>[2x]MRVLGIETSCDETGIAIYDDEKGLLANQLYSQVKLHADYGGVVPELASRDHVRKTVPLIQAALKESGLTAKDIDAVAYTAGPGLEGALLVGATVGRSLAFAWDVPAIPVHHMEGHLLAPMLEDNPPEFPFVALLVSGGHTQLISVTGIGQYELLGESIDDAAGEAFDKTAKLLGLDYPGGPLLSKMAAQGTAGRFVFPRPMTDRPGLDFSFSGLKTFAANTIRDNGTDDQTRADIARAFEDAVVDTLMIKCKRALDQTGFKRLVMAGGVSANRTLRAKLAEMMKKRRGEVFYARPEFCTDNGAMIAYAGMVRFKAGATADLGVSVRPRWPLAELPAAHHHHHH;>[2x]MRILAIDTATEACSVALWNDGTVNAHFELCPREHTQRILPMVQDILTTSGTSLTDINALAYGRGPGSFTGVRIGIGIAQGLALGAELPMIGVSTLMTMAQGAWRKNGATRVLAAIDARMGEVYWAEYQRDENGIWHGEETEAVLKPEIVHERMQQLSGEWVTVGTGWQAWPDLGKESGLVLRDGEVLLPAAEDMLPIACQMFAEGKTVAVEHAEPVYLRNNVAWKKLPGKEHHHHHH

The N6-threonylcarbamoyladenosine (t6A) modification at position 37 of ANN-decoding tRNAs is one of the few modifications that are found in the three domains of life. In the first half of the reaction, YrdC utilizes ATP, L-threonine and bicarbonate to synthesize an unstable intermediate TCA, whose threonylcarbamoyl-moiety is subsequently transferred onto the adenosine at position 37 of the substrate tRNAs by the cooperative action of three proteins YeaZ, YgjD and YjeE. In archaea and yeast, the transfer reaction requires the kinase, putative endopeptidase and other proteins of small size (KEOPS) protein complex, composed of Kae1, Bud32, Cgi121 and Pcc1, complemented by a fifth fungi-specific protein Gon7 in yeast. It is now well established that YgjD and its orthologs Kae1 and Qri7 are responsible for the catalysis of the transfer reaction. YgjD and YeaZ are forming a heterodimer that is capable of interacting with YjeE.

We wanted to test the pertinence of the ADP bound at the YgjD–YeaZ interface using two mutants, YeaZR118A and YgjDV85E. The crystal structure of YgjDV85E–YeaZ in the presence of ATP showed no ADP-like electron density at the dimer interface. The mutations of two residues that contact this ADP molecule (YeaZR118A and YgjDV85E) did not confer any effect on the heterodimerization of YgjD and YeaZ, nor on the activation of the ATPase activity of YjeE. The ATPase activity of the ternary YgjDV85E–YeaZ–YjeE and YgjD–YeaZR118A–YjeE complexes remained unaffected and the latter is fully active for the in vitro biosynthesis of t6A.>[2x]GELVRTDSPNFLCSVLPTHWRCNKTLPIAFKVVAKGDVPDGTLVTVMAGNDENYSAELRNATAAMKNQVARFNDLRFVGRSGRGKSFTLTITVFTNPPQVATYHR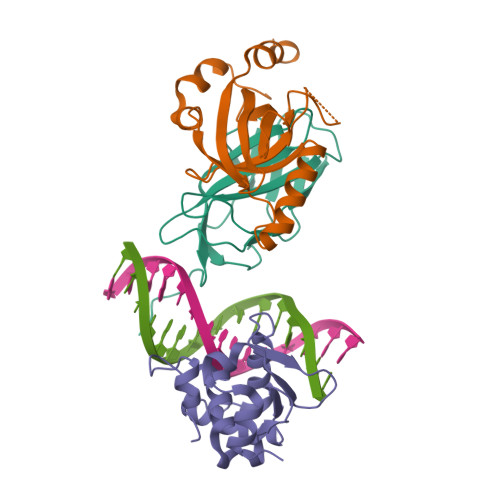AIKITVDGPREPRRHRQKLDDQTKPGSLSFSERLSELEQLRRTAMRVSPHHPAPTPNPRASLNHSTAFNPQPQSQMQDARQIQPSPPWSYDQSYQYLGS;>[2x]MPRVVPDQRSKFENEEFFRKLSRECEIKYTGFRDRPHEERQTRFQNACRDGRSEIAFVATGTNLSLQFFPASWQGEQRQTPSREYVDLEREAGKVYLKAPMILNGVCVIWKGWIDLHRLDGMGCLEFDEERAQQEDALAQQA;>[2x]SLQRVPSYDSFDSEDYPAALPNHKPKGTFKDYVRDRADLNKDKPVIPAAALAGYTGSGPIQLWQFLLELLTDKSCQSFISWTGDGWEFKLSDPDEVARRWGKRKNKPKMNYEKLSRGLRYYYDKNIIHKTAGKRYVYRFVCDLQSLLGYTPEELHAMLDVKPDADE>[2x]CPRFLKVKNWETDVVLTDTLHLKSTLETGCTEHICMGSIMLPSQHTRKPEDVRTKDQLFPLAKEFLDQYYSSI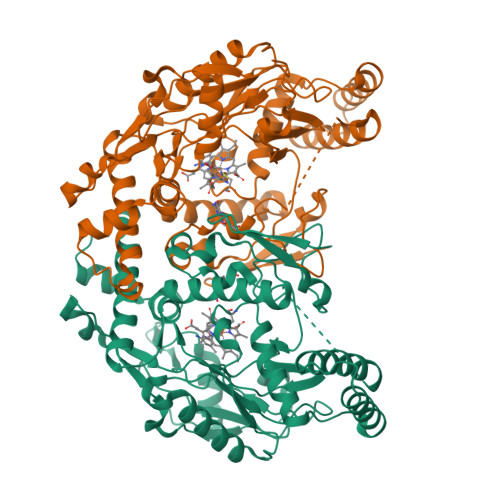KRFGSKAHMDRLEEVNKEIESTSTYQLKDTELIYGAKHAWRNASRCVGRIQWSKLQVFDARDCTTAHGMFNYICNHVKYATNKGNLRSAITIFPQRTDGKHDFRVWNSQLIRYAGYKQPDGSTLGDPANVQFTEICIQQGWKAPRGRFDVLPLLLQANGNDPELFQIPPELVLEVPIRHPKFDWFKDLGLKWYGLPAVSNMLLEIGGLEFSACPFSGWYMGTEIGVRDCCDNSRYNILEEVAKKMDLDMRKTSSLWKDQALVEINIAVLYSFQSDKVTIVDHHSATESFIKHMENEYRCRGGCPADWVWIVPPMSGSITPVFHQEMLNYRLTPSFEYQPDPWNTHVWKG Beta2-glycoprotein I (β2GPI) is the major target for autoimmune antibodies associated with antiphospholipid syndrome (APS), an autoimmune disease characterized clinically by thrombosis and recurrent pregnancy loss. The binding sites for anionic phospholipids, lipoprotein receptors (including ApoER2) and GPIb are in domain V of β2GPI (β2GPI-DV). Circular β2GPI can be converted to an extended form by altering pH and salt concentrations, binding to a high-affinity antibody directed to domain I or by the binding to cardiolipin. β2GPI, which is abundant in plasma (about 170 µg/ml or 4 µM), acquires its prothrombotic properties only in the presence of anti-β2GPI antibodies. Anti-β2GPI antibodies create multivalent β2GPI/anti-β2GPI complexes that have pathological properties compared to pathologically inactive β2GPI monomers, which are normally present in plasma.

β2GPI binds anionic phospholipids and the A1 modules by its domain V. In the crystal structures of a full-length β2GPI in the extended conformation, domain V forms essentially no contacts with the adjacent domain. There are no glycosylation sites in β2GPI that could affect function of domain V indicating that the individual domain V (β2GPI-DV) dissected from the full-length β2GPI will function as domain V in the extended form of β2GPI. We solved the crystal structure of the isolated domain V to 1.9 Å resolution. As illustrated by Figure 6, the backbone conformation of β2GPI-DV is nearly identical to the structure of this domain in the full-length β2GPI. The largest difference between the structures is localized to a C-terminal loop. Experimental data strongly suggests that this loop is flexible in the native protein. Also, the residues in the loop are either weak or missing from the NMR spectrum of β2GPI-DV in solution reflecting its internal flexibility. The structural similarity between β2GPI-DV and domain V in the full-length β2GPI provides convincing evidence that the isolated recombinant β2GPI-DV mimics domain V in the extended form of β2GPI. We have previously demonstrated that the A1 module binds to the C-terminal part of β2GPI-DV and, therefore, the N-terminal peptide tag on β2GPI-DV and the bound anti-tag antibody will not interfere with the binding of the A1 modules to β2GPI-DV. The concentration of A1 at half-maximal inhibition was 176±37 µM for β2GPI in serum and 188±44 µM for domain V. This observation demonstrates that A1 binds circular and extended β2GPI with the same affinity suggesting that the binding site for A1 is not obscured in the circular form of β2GPI.

>GSCKLPVKKATVVYQGERVKIQEKFKNGMLHGDKVSFFCKNKEKKCSYTEDAQCIDGTIEVPKCFKEHSSLAFWKTDASDVKPCA[2x]>MIFSVDKVRADFPVLSREVNGLPLAYLDSAASAQKPSQVIDAEAEFYRHGYAAVHRGIHTLSAQATEKMENVRKRASLFINARSAEELVFVRGTTEGINLVANSWGNSNVRAGDNIIISQMEHHANIVPWQMLCARVGAELRVIPLNPDGTLQLETLPTLFDEKTRLLAITHVSNVLGTENPLAEMITLAHQHGAKVLVDGAQAVMHHPVDVQALDCDFYVFSGHKLYGPTGIGILYVKEALLQEMPPWEGGGSMIATVSLSEGTTWTKAPWRFEAGTPNTGGIIGLGAALEYVSALGLNNIAEYEQNLMHYALSQLESVP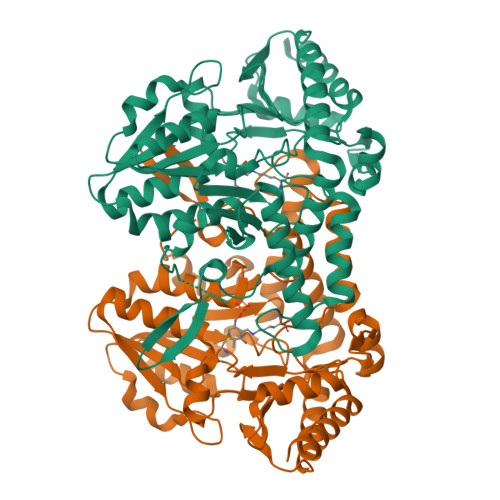DLTLYGPQNRLGVIAFNLGKHHAYDVGSFLDNYGIAVRTGHHCAMPLMAYYNVPAMCRASLAMYNTHEEVDRLVTGLQRIHRLLG[2x]> MGHHHHHHMLHLLEQIRAYCETCWEWQEAHEPGMDQDKNPMPAPVEHQICPAVCVLMKLSFDEEHRHAMNELGGLQAIAELLQVDCEMYGLTNDHYSITLRRYAGMALTNLTFGDVANKATLCSMKGCMRALVAQLKSESEDLQQVIASVLRNLSWRADVNSKKTLREVGSVKALMECALEVKKESTLKSVLSALWNLSAHCTENKADICAVDGALAFLVGTLTYRSQTNTLAIIESGGGILRNVSSLIATNEDHRQILRENNCLQTLLQHLKSHSLTIVSNACGTLWNLSARNPKDQEALWDMGAVSMLKNLIHSKHKMIAMGSAAALRNLMANRPAKYKDANIMSPGSSLPS;> LTGCGDIIAEQ

Adenomatous polyposis coli (APC) is an important human tumor suppressor protein which plays critical roles in diverse cellular processes such as Wnt/β-catenin signaling, cell adhesion, cell migration, mitosis and chromosomal instability, and so on. The N-terminal armadillo repeat (ARM) domain of APC is the most conserved region among its vertebrate and invertebrate homologs, and mediates its association with a variety of binding partners including APC membrane recruitment 1 (Amer1, also named as WTX for ‘Wilms tumor gene on the X chromosome’), Asef, Sam68, and IQGAP1. By recruiting APC to the plasma membrane, Amer1 regulates the APC-dependent maintenance of intercellular junctions. In addition, together with APC and Axin, Amer1 promotes ubiquitination and degradation of β-catenin, thus negatively regulates the Wnt signal transduction pathway.

Intriguingly, ITC experiments demonstrated that peptides of Amer1-A1 (residues 325–335) and -A2 (residues 496–508) sequences exhibited approximately equal binding affinities for APC–ARM as full Amer1-A1 (residues 280–368) and -A2 (residues 380–531), respectively. Therefore, Amer1 residues 325–335 and 496–508 are regarded to represent the core A1 and A2 fragments for APC binding, respectively, although other conserved Amer1 residues nearby such as residues 315–324 may also contribute to the interaction with APC. To further understand the molecular basis of how APC recognizes Amer1, we determined the crystal structures of the APC–ARM/Amer1-A1, APC–ARM/Amer1-A2, and APC–ARM/Amer1-A4 complexes to 1.90 Å, 2.00 Å, and 1.70 Å resolutions, respectively. Despite possessing apparently different sequences, Amer1-A1, -A2, and -A4 adopt remarkably similar conformations when bound to APC–ARM, both in anti-parallel manners with respect to the armadillo repeats of APC. At all three interfaces between APC–ARM and Amer1-A1/A2/A4, four highly conserved asparagine residues, N507/N550/N594/N641 from the H3 helices of armadillo repeats 2/3/4/5 of APC–ARM function as rivets fastening Amer1-A1/A2/A4 onto its surface groove. In addition, two basic residues, APC-K516 and -R549, straddle the middle portion of Amer1-A1/A2/A4 peptides on both sides. They form salt bridges with a conserved acidic residue A1-D330/A2-D503/A4-E370 and make hydrogen bonds with the main chain carbonyl groups of A1-C328/A1-G329/A2-S501/A2-G502/A4-G368. Moreover, two tryptophan residues, APC-W593 and -W553, provide more binding affinity by hydrogen bonding with A1-T326/A2-S499 and making van der Waals interactions with A1-G327/A1-G329/A2-Y500/A2-G502/A4-G367/A4-G369, respectively. Furthermore, substitution of the crucial hydrophobic residue APC-F510 by a lysine reduced the complex formation between APC–ARM and Amer1-A1.(3R,4R,5R)-3,4-dihydroxy-5-({[(1R)-2-hydroxy-1-phenylethyl]amino}methyl)pyrrolidin-2-one 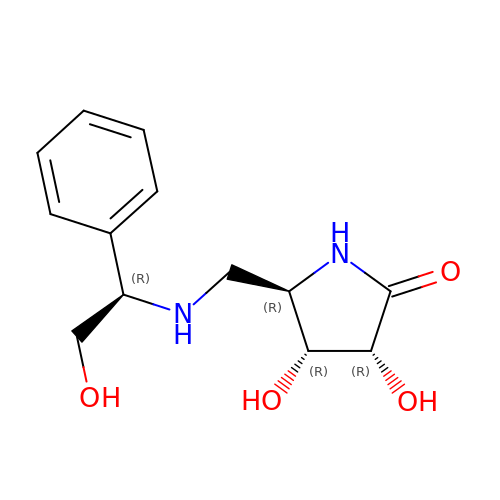| C13 H18 N2 O4 | KRKSNZJFCXFNFF-WRWGMCAJSA-N> ATTQIGEIVKTVANTVESEIKAELGVIPSLNAVETGATSNTEPEEAIQTRTVINMHGTAECLVENFLGRSALVCMRSFEYKNHSTSTSSIQKNFFIWTLNTRELVQIRRKMELFTYLRFDTEITIVPTLRLFSSSNVSFSGLPNLTLQAMYVPTGARKPSSQDSFEWQSACNPSVFFKINDPPARLTIPFMSINSAYANFYDGFAGFEKKATVLYGINPANTMGNLCLRVVNSYQPVQYTLTVRVYMKPKHIKAWAPRAPRTMPYTNILNNNYAGRSAAPNAPTAIVSHRSTIKTMPNDINLTTA;> SPSAEACGYSDRVLQLKLGN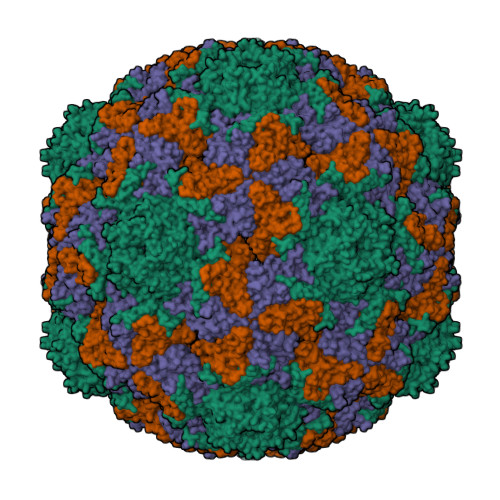SSIVTQEAANICCAYGEWPTYLPDNEAVAIDKPTQPETSTDRFYTLKSKKWESNSTGWWWKLPDALNQIGMFGQNVQYHYLYRSGFLCHVQCNATKFHQGTLLIVAIPEHQIGKKGTGTSASFAEVMKGAEGGVFEQPYLLDDGTSLACALVYPHQWINLRTNNSATIVLPWMNSAPMDFALRHNNWTLAVIPVCPLAGGTGNTNTYVPITISIAPMCAEYNGLRNAITQ;> GVPTCLLPGSNQFLTTDDHSSAPAFPDFSPTPEMHIPGQVHSMLEIVQIESMMEINNVNDASGVERLRVQISAQSDMDQLLFNIPLDIQLEGPLRNTLLGNISRYYTHWSGSLEMTFMFCGSFMTTGKLIICYTPPGGSSPTDRMQAMLATHVVWDFGLQSSITIIIPWISGSHYRMFNTDAKAINANVGYVTCFMQTNLVAPVGAADQCYIVGMVAAKKDFNLRLMRDSPDIGQSAILPEQ>[2x]GGAAGUGUACCUAGGGAUCCACCUCG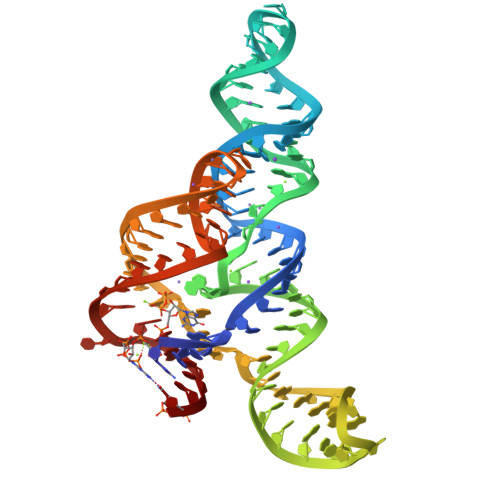AGAGAGGAAGGACCAAGCGGUACAGGCCUACUUCGGUAGGUUACACCGUGGGGAUAAAAGACCCGUGGCAAGUUUC>MNLPTAQEVQGLMARYIELVDVGDIEAIVQMYADDATVENPFGQPPI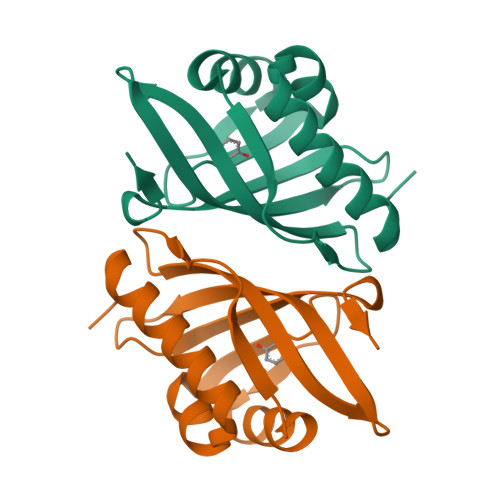HGREQIAAFYRQGLGGGKVRACLTGPVRASHNGCGAMPFRVEMVWNGQPCALDVIDVMRFDEHGRIQTMQAYWSEVNLSVREPQ[4x]> MTLVPDLTATDLARHRWLTDNSWTRPTWTVAELEAAKAGRTISVVLPALNEEETVGGVVETIRPLLGGLVDELIVLDSGSTDDTEIRAMAAGARVISREVALPEVAPQPGKGEVLWRSLAATTGDIIVFIDSDLIDPDPMFVPKLVGPLLLSEGVHLVKGFYRRPLKTSGSEDAHGGGRVTELVAR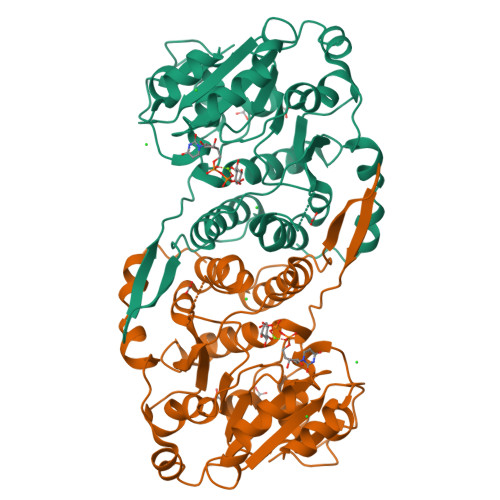PLLAALRPELTCVLQPLGGEYAGTRELLMSVPFAPGYGVEIGLLVDTYDRLGLDAIAQVNLGVRAHRNRPLTDLAAMSRQVIATLFSRCGVPDSGVGLTQFFADGDGFSPRTSEVSLVDRPPMNTLRGKLAAALEHHHHHH>[4x]ATQGVFTLPANTRFGVTAFANSS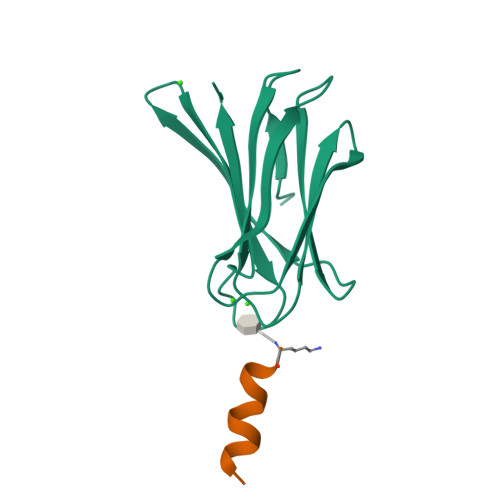GTQTVNVLVNNETAATFSGQSTNNAVIGTQVLNSGSSGKVQVQVSVNGRPSDLVSAQVILTNELNFALVGSEDGTDNDYNDAVVVINWPLG;>[4x]KYKKALKKLAKL> EQSSSEIKIVRDEYGMPHIYANDTWHLFYGYGYVVAQDRLFQMEMARRSTQGTVAEVLGKDFVKFDKDIRRNYWPDAIRAQIAALSPEDMSILQGYADGMNAWIDKVNTNPETLLPKQFNTFGFTPKRWEPFDVAMIFVGTMANRFSDSTSEIDNLALLTALKDKYGVSQGMAVFNQLKWLVNPSAPTTIAVQESNYPLKFNQQNSQTA;> SNMWVIGKSKAQDAKAIMVNGPQFGWYAPAYTYGIGLHGAGYDVTGNTPFAYPGLVFGHNGVISWGSTAGFGDDVDIFAERLSAEKPGYYLHNGKWVKMLSREETITVKNGQAETFTVWRTVHGNILQTDQTTQTAYAKSRAWDGKEVASLLAWTHQMKAKNWQEWTQQAAKQALTINWYYADVNGNIGYVHTGAYPDRQSGHDPRLPVPGTGKWDWKGLLPFEMNPKVYNPQSGYIANWANSPQKDYPASDLFAFLWGGADRVTEIDRLLEQKPRLTADQAWDVIRQTSRQDLNLRLFLPTLQAATSGLTQSDPRRQLVETLTRWDGINLLNDDGKTWQQPGSAILNVWLTSMLKRTVVAAVPMPFDKWYSASGYETTQDGPTGSLNISVGAKILYEAVQGDKSPIPQAVDLFAGKPQQEVVLAALEDTWETLSKRYGNNVSNWKTPAMALTFRANNFFGVPQAAAEETRHQAEYQNRGTENDMIVFSPTTSDRPVLAWDVVAPGQSGFIAPD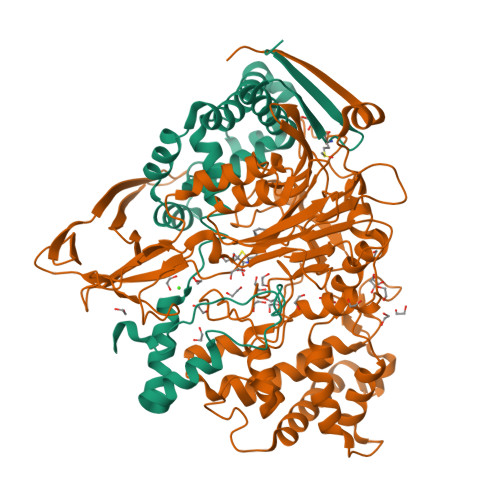GTVDKHYEDQLKMYENFGRKSLWLTKQDVEAHKESQEVLHVQR> MAISIKTPEDIEKMRVAGRLAAEVLEMIEPYV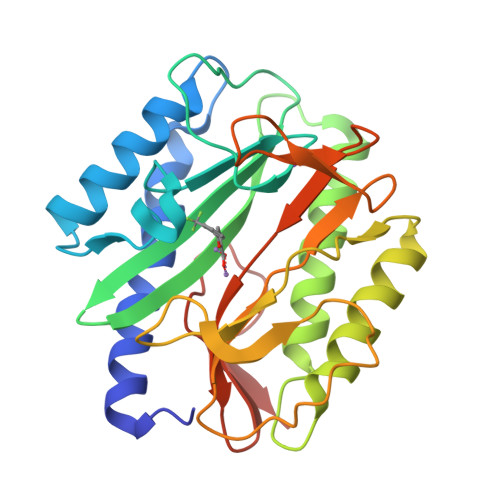KPGVSTGELDRICNDYIVNEQHAVSACLGYHGYPKSVCISINEVVCHGIPDDAKLLKDGDIVNIDVTVIKDGFHGDTSKMFIVGKPTIMGERLCRITQESLYLALRMVKPGINLREIGAAIQKFVEAEGFSVVREYCGHGIGRGFHEEPQVLHYDSRETNVVLKPGMTFTIEPMVNAGKKEIRTMKDGWTVKTKDRSLSAQYEHTIVVTDNGCEILTLRKDDTIPAIISHDE>TGTANTLFGTASTGTSLFSSQNNAFAQNKPTGFG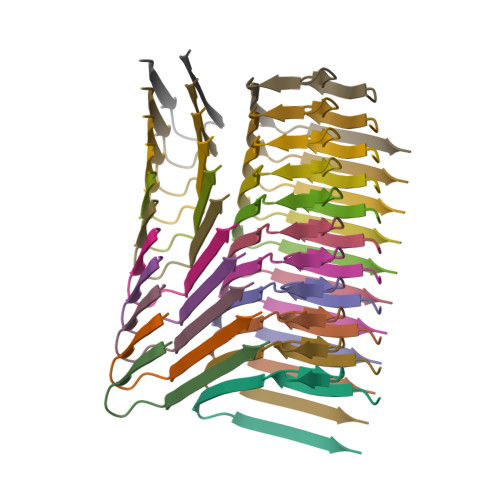NFGTST[22x]>MVKVDLESKRYGEKLKEVFLMLDNNVVECIKEITESSRNGKLVFFVGAGVSTLSDYPQWWRLVDKYHEELYGSPKKGNYSSDEYLRIPQIFYNVKGEMAFDGILKDFFQVDKPTNPIHDKILAMNPAHVITTNYDNLIDTACWKRGKYFSVISAEEDVANATSSRYLLKVAGDFRKGFKGENVVLKEDDYLNYDQNYPLISNLMKTIIATHTIVFIGYGLGDYNINMLLNWVRKLQKDSFHKPFFIRTDPSPIENETLIYYENKGLRIIDAASLIDSNEYDYLERYSAVMDLLIESQENKFITKDDEVIDYIYGKISPLFALQYIRKIDLKHVFEYDYHFEVNGTVVRHKNKGFGYMERFFELKESCDERSKLSKKQYERFNALFNFFEKNGVICMAKDAGTLNTSIEINSLAYHGKYDVMKKFIEEQSVSIEDDYKKAFFLACLGRWEESYDLYSNIILNSIDESNGCVYYLSQINRYRIYQSITQAVTQFNGLGLLTFGRHYKPFTDEFLARIEREMTNFNIDDLFNGMPFEFQKKYKILEFLSDNQFLYDDTVKLFELTNKVRSEMSEGSYSFGMSSDIVVLLRLYDNLRFLYENCLWSVSFHEFHQYIRNSMSLLIEKAEYERTRDIDELGFSFFGKKSGFFMEYYDFVNISRHFKIDDIKNLERSCSIDKIRFGEQEKIEEYLVGIAEEITKQFSANGMNVVFYTQFISEAKAALYFAKYVKLSEEGLGKIVKALLFYFPERDLDIGKRYVWLERLTKCNELPKSIISIIDDFLVLQAEKHIDQNYSEVSSNGLYSRDYGALIKHFEKNFISKRLSEITLCLTQDKQKQIDFLFKLLPLLSTNAKSHLLSFKSVENINDLMNGIRIGLIDEFTPEHEELIIEYLETRKVNYIVEKEKGIQTFSSNDYMSTFGIWYFLEEINNSKMEEFIGMDDQYDFFVDPENFDYKKFIPSWLKNYNDKLLGKIAGNKHMKHHVIEVLKERVKNSNDKRYLEILMNYFI[4x]

As a sirtuin (SIR2) family protein, defense-associated sirtuin2 (DSR2) has been demonstrated to participate in bacterial anti-phage resistance via depleting nicotinamide adenine dinucleotide (NAD+) of infected cells, which can be activated by tail tube protein (TTP) and inhibited by DSR anti-defense 1 (DSAD1) of diverse phages. To defend phage invasion, Bacillus subtilis utilizes DSR2 proteins to sense and recognize phage SPR tail tube protein (TTP), then unleashes NADase activity of its SIR2 domain to deplete the cell of NAD+ and abort phage propagation during infection. Each DSR2 protomer contains three domains, an N-terminal SIR2 domain (SIR2, residues 1 to 297), a middle connector domain (MID, residues 297 to 627), and a C-terminal sensor domain (CTD, residues 627 to 1005). Structural analyses and biochemical studies reveal that DSR2 forms a tetramer with a SIR2 central core and two distinct conformations.

The cryo-EM structures of DSR2 from B. subtilis 29R were determined in its apo form at 2.92 Å and its complexed form with TTP and DSAD1 at 3.16 Å and 2.98 Å, respectively. The final models contain only partial tetramer including two complete protomers DSR2A and DSR2B, and two SIR2 domains of DSR2C-SIR2 and DSR2D-SIR2 due to its instability. In the structure, four N-terminal SIR2 domains form a central core consisting of two SIR2 dimers via a head-to-head arrangement with a buried interface area of ~1700 Å2. The complete protomer DSR2A and DSR2B form a scissors-like dimer with a total buried area of ~4000 Å2. Further conformational comparison indicates substantial difference between DSR2A/open and DSR2B/closed with a root mean square deviation (RMSD) of 2.800 Å. Besides the abovementioned identifiable α42, another obvious difference exists in the loop (α30-α31 loop, residues 633 to 643) of CTD with a ~9-Å displacement between two protomers when superimposed. In addition, the small triangular protruding module of SIR2 domain has a conformational change with a rotation of ~20° and a translation of ~7 Å. The result indicates that DSR2 lacks the capacity to catalyze NAD+ hydrolysis alone, suggesting a potential self-inhibitory property of apo DSR2. In addition, the active site suggests that residues N133 and H171 are crucial for DSR2 NADase activity. In vitro NADase assays further confirm both mutants of N133A and H171A aborting the NADase activity, which is consistent with the result of previously reported phage infection analyses.Cyclodipeptide synthases (CDPS) are a family of tRNA dependant enzymes that synthesise cyclic dipeptides using two aminoacylated tRNA (aa-tRNA) as substrates. Here, we investigated a CDPS from Bacillus thermoamylovorans (BtCDPS), a cLL-synthesising enzyme that utilises Leu-tRNALeu as a substrate, and is predicted to be part of the biosynthetic machinery involved in pulcherrimin biosynthesis. The aminoacyl moiety of tRNA is transferred onto the conserved active site serine residue (S33 in BtCDPS), forming an aminoacyl-enzyme intermediate. This intermediate then reacts with a second aa-tRNA to form a dipeptidyl-enzyme intermediate, which undergoes intramolecular cyclisation aided by a conserved tyrosine residue to form a cyclic dipeptide.

The crystal structure of full-length (residues 1–232) and S33A mutant enzymes was solved at a resolution of 1.69 Å and 1.78 Å, respectively (ESI†). BtCDPS has a single domain with an αβ fold similar to other CDPS. The structure of CDPS is highly similar to yvmC-BLIC (RMSD 0.88 Å, over 212 residues), AlbC (RMSD 2.25, over 212 residues) and Rv2275 (RMSD 2.00 Å, over 199 residues). A molecule of 1,2-hexanediol co-crystallised in the P1 binding pocket adjacent to the catalytic residues. Binding is facilitated by a hydrogen bond contact with the side chain carboxyl group of the catalytic Glu179 residue and other non-bonding contacts with P1 pocket residues. The aliphatic chain of 1,2-hexanediol molecule is projected deep into the P1 pocket, which is lined with mainly hydrophobic residues (L29, G31, L61, A63, F112, Phe182, F183, L197), ideal to accommodate a leucine substrate. However, the P2 pocket is far shallower and more solvent exposed. The P2 pocket is lined with a mixture of residues (R201, W203, K204, D148, S152, A149, R153), which is in keeping with the previously reported sequence homology that suggests the P2 pocket has conserved Met, Trp and Ala residues. The side chain of R153 is projected into the active site and makes a strong hydrogen-bond (distance = 2.6 Å) with the hydroxyl side chain of the catalytic serine residue, which is unknown for this class of enzymes. Moreover, the positioning of R153 makes it an ideal candidate to interact with the 5′-phosphate group of the aa-AMP moiety of tRNA substrate.

> GMQQVIKDLFYVVPLSRNCEKIYKNKTHILLGISPFNSKFSQNYIHQLIDWSSKNFKNVTVLLAGDEAKNLLEALGTPTTKAERKVRKEIRRHFRFSEEALRKNGREIDIYTFSDFKNNKIYNEVYQNVIYYFEKDEKFRKSCLAMSHDALSSRAKSLNMEDIEITDNMLFHAVKYVLAELPFFLSGASILGYKESVLAYHRPWKLGEKIKNSEFYIKMSDNQGYIILKQIN>[2x]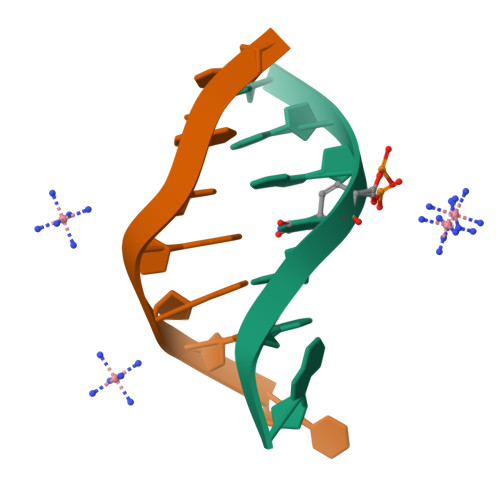GCGTGCG;>[2x]CGCACGC> MTKIYRCKLTLHDNVFFASREMGILYETEKYFHNWALSYAFFKGTIIPHPYGLVGQNAQTPAYLDRDREQNLLHLNDSGIYVFPAQPIHWSYQINTFKAAQSAYYGRSVQFGGKGATKNYPINYGRAKELAVGSEFLTYIVSQKELDLPVWIRLGKWSSKIRVEVEAIAPDQIKTASGVYVCNHPLNPLDCPANQQILLYNRVVMPPSSLFSQSQLQGDYWQIDRNTFLPQGFHY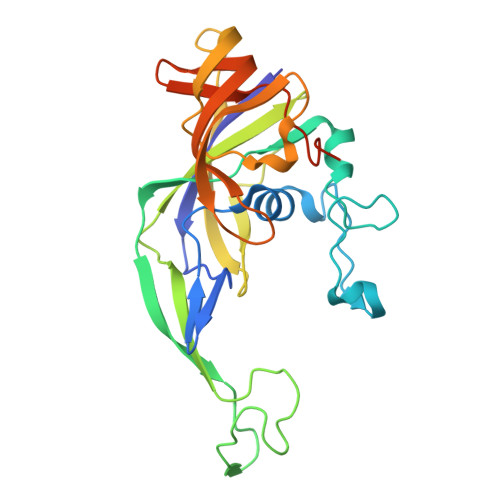GATTAIAQDSPQLSLLDTN CEP192 and CEP44 are proteins with a key role in centrosome and centriole biogenesis. We have recently determined the structures of the N-terminal Calponin Homology (CH) domain of human CEP44 and the so-called Spd2 domain of human CEP192. Both structures were obtained through X-ray crystallography at a resolution of 2.3 and 2.1 Å, respectively, and were experimentally phased. The N-terminal domain of CEP44 shares a weak sequence similarity to various CH domains, most of which members of the IFT81/NDC80/Hec families, whereas the Spd2 domain retrieves sequence matches to members of the PapD-like superfamily.

In contrast, CEP192 is an essential component of the pericentriolar material (PCM), a proteinaceous matrix that surrounds centrioles in which CEP192 exerts a scaffolding and regulatory function. The common isoform of human CEP192 is 2537 residues long and a sequence analysis of its C-terminal part suggests the presence of eight tandem domains that are similar to members of the PapD-like superfamily. The human CEP192 domains 4 and 5 constitute the so-called Spd2 domain that is ubiquitously present in all SPD2/CEP192 homologues and represents the most conserved region amongst them. Its highest sequence conservation is found in two motifs, as judged by multiple sequence alignment of orthologous sequences: Motif 1 (PLXGYGG) located at the C-terminal end of domain 4, and Motif 2 (GDEXXR) located within domain 5. The crystal structure of the human Spd2-domain revealed two seven-stranded Ig-like β-sandwiches with distinctive kinks (β-a1/ β-a2 and β-c’1/ β-c’2) at the edges, a feature that is characteristic for the PapD-like superfamily. The two constituent domains pack together to form an extended cradle-like structure. The two highly conserved motifs PLXGYGG and GDEXXR define the interface between both domains via an extensive network of interactions. Intriguingly, Motif 2 is found within a large (60 residue) insertion that precedes the C-terminal β-strand g of domain 5 and consists of a helix (α1) and an irregular part that wraps around it before proceeding to complete domain 5. This insertion defines a unique feature that is essential for maintaining the cradle-like conformation of the Spd2 domain. The comparison of the Spd2 crystal structure with the AF2 predicted model (AF-Q8TEP8-F1-model_v1) revealed striking similarity with 273 structurally equivalent residues superposed with rmsd of 1.83 Å.

> GPKGEVISSGSKPLSPGPCLDIPSILSNKQFLAWGGVPLGRTQLQKLALRNNSASTTQHLRLLIRGQDQDCFQLQNTFGSEQRLTSNCEIRIHPKEDIFISVLFAPTRLSCMLARLEIKQLGNRSQPGIKFTIPLSGYGGTSNLILEGVKKLSDSYMVTVNGLVPGKESKIVFSVRNTGSRAAFVKAVGFKDSQKKVLLDPKVLRIFPDKFVLKERTQENVTLIYNPSDRGINNKTATELSTVYLFGGDEISRQQYRRALLHKPEMIKQILPEHSVLQNINFVEAFQDELLVTEVYDLPQRPNDVQLFYGSMCKIILSVIGEFRDCISSREFLQPSSKASLESTSDLGASGK N-{5-[4-(4-METHYLPIPERAZIN-1-YL)PHENYL]-1H-PYRROLO[2,3-B]PYRIDIN-3-YL}NICOTINAMIDE 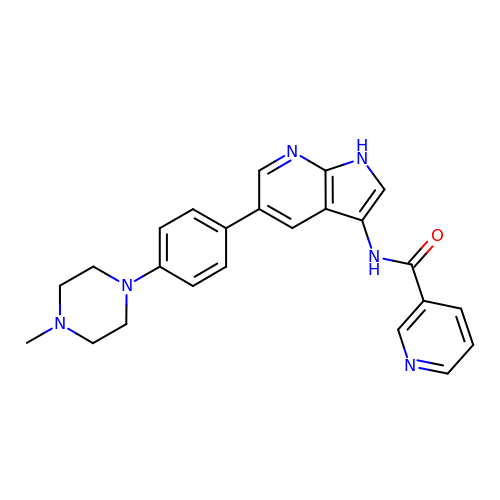| C24 H24 N6 O | YJWJKKXGAPWLGT-UHFFFAOYSA-N>[3x]MFKTIANDAYRENNHTKKLLVLVVGETARAANYSLGGYTKNDTNFYTKKDNVVFFDNFSSCGTATAVSLPCMFSISKRENYSSSEFQENAMDVLYKTGVDAAWFDNNSGGCKGVCDRLAYKQKLSSDLDENLL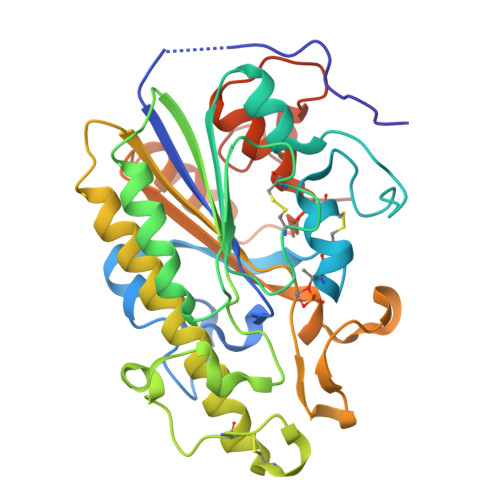IPFKEKLNHLSDQNIIVLHLQGSHGPTYYKRYPSEFKKFTPTCDTNELSKCDSEALINTYDNTLLYTDYLLSEIIKLLKEQKSYESSLFYLSDHGESLGENGIYLHGMPYAIAPSYQTHIPAIFWSNDEKLMNLAKEHKGLKLSQDNLFSTLLGYFNVKTSVYEPEYDLLNPKLKANPGGGGGGHHHHHHHH> MIERILEFTAKHEEWIVGENVEDFTNENIAMFLSRVSN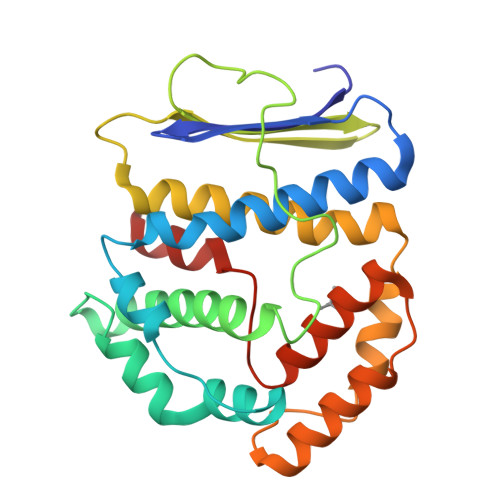TVSSKIPGYLGEKIDVNGLLSIKIEGSLEEKLKALISPKVSRQIGRLVMEDDKKLKKLLVEVAKAVLTREILKNELPIEFPGGKIEGLKIQPRYEEDHINFTARYGSWIVVKRMIIDEKTPLLDIARLLASINETAVNKIKDFADVDDKKIVEYFGGFKKVKKEEEIKEIVQLFREFKGNEFEVRYAAREMLSKLGLKVDVPSKNLEKYLEKAG> FQSNAMFAWWGRTVYQFRYIVIGVMVALCLGGGVYGISLGNHVTQSGFYDEGSQSVAASLIGDEVYGRDRTSHVVAILTPPDDKKVTDKAWQKKVTEELDQVVKDHEDQIVGWVGWLKAPDTTDPTVSAMKTQDLRHTFISIPLQGDDDDEILKNYQVVEPELQQVNGGDIRLAGLNPLASELTGTIGEDQKRAEVAAIPLVAVVLFFVFGTVIAAALPAIIGGLAIAGALGIMRLVAEFTPVHFFAQPVVTLIGLGIAIDYGLFIVSRFREEIAEGYDTEAAVRRTVMTSGRTVVFSAVIIVASSVPLLLFPQGFLKSITYAIIASVMLAAILSITVLAAALAILGPRVDALGVTTLLKIPFLANWQFSRRIIDWFAEKTQKTKTREEVERGFWGRLVNVVMKRPIAFAAPILVVMVLLIIPLGQLSLGGISEKYLPPDNAVRQSQEQFDKLFPGFRTEPLTLVMKREDGEPITDAQIADMRAKALTVSGFTDPDNDPEKMWKERPANDSGSKDPSVRVIQNGLENRNDAAKKIDELRALQPPHGIEVFVGGTPALEQDSIHSLFDKLPLMALILIVTTTVLMFLAFGSVVLPIKAALMSALTLGSTMGILTWMFVDGHGSGLMNYTPQPLMAPMIGLIIAVIWGLSTDYEVFLVSRMVEARERGMSTAEAIRIGTATTGRLITGAALILAVVAGAFVFSD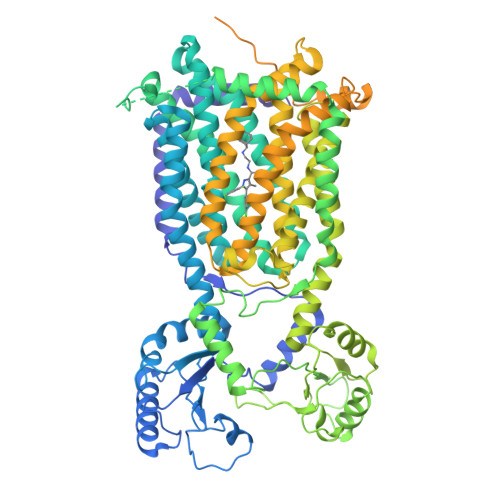LVMMKYLAFGLLIALLLDATIIRMFLVPAVMKLLGDDCWWAPRWMKRVQEKLGLGETELPDERKRPTVRESETDQRALVGVGAPPPPPRPHDPTHPAPEPVRPMPPMRSNAPSAAGTARISTPPQPPQPPQAPAQQAGDEPATTRFAMARNAVRNAVNSAVHGGAGSAAAPTERAPRPGGPAQPPAPPQREEREIESWLGALRGPAPAKNVPQPPAQPQRPSTDTTRAMPPQGRPPAGPADRGNENAPTTAFSAQRPPNGGAPADATTAIPTPPQREQEPSTEKLNTREDAPEDPETKRRGGGMSAQDLLRREGRL> GDPVEDIIHDALGNTARRAISSATNVESAANTTPSSHRLETGRVPALQAAETGATSNATDENMIETRCVVNRNGVLETTINHFFSRSGLVGVVNLTDGGTDTTGYATWDIDIMGFVQLRRKCEMFTYMRFNAEFTFVTTTENGGARPYMLQYMYVPPGAPKPTGRDAFQWQTATNPSVFVKLTDPPAQVSVPFMSPASAYQWFYDGYPTFGQHPETSNTTYGLCPNNMMGTFAVRVVSREASQLKLQTRVYMKLKHVRAWVPRPIRSQPYLLKNFPNYDSSKITNSARDRSSIKQANM;> SPSVEACGYSDRVAQLTVGNSSITTQEAANIVLAYGEWPEYCPDTDATAVDKPTRPDVSVNRFYTLDSKMWQENSTGWYWKFPDVLNKTGVFGQNAQFHYLYRSGFCLHVQCNASKFHQGALLVAVIPEFVIAGRGSN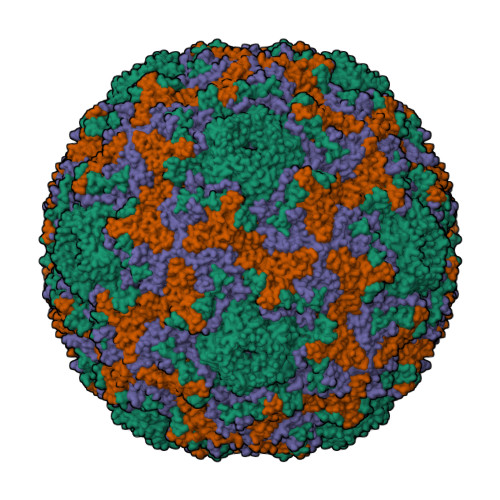TKPNEAPHPGFTTTFPGTTGATFYDPYVLDSGVPLSQALIYPHQWINLRTNNCATVIVPYINAVPFDSAINHSNFGLIVIPVSPLKYSSGATTAIPITITIAPLNSEFGGLRQAVSQ;> GIPAELRPGTNQFLTTDDGTAAPILPGFTPTPTIHIPGEVHSLLELCRVETILEVNNTTEATGLTRLLIPVSSQNKADELCAAFMVDPGRIGPWQSTLVGQICRYYTQWSGSLKVTFMFTGSFMATGKMLVAYSPPGSAQPANRETAMLGTHVIWDFGLQSSVSLVIPWISNTHFRTAKTGGNYDYYTAGVVTLWYQTNYVVPPETPGEAYIIAMGAAQDNFTLKICKDTDEVTQQAVLQ;> MGAQVSTQKSGSHETGNVATGGSTINFTNINYYKDSYAASATRQDFTQDPKKFTQPVLDSIRELSAPLN>MKIIALRSSLKLAARIAEELKTEPVMPDERRFPDGELYLRYDEDLTGHNIFIIGNTHSDAEVMEMILTLSAIQDYRTKSVNIIAPYYGYARQHQRYKNGEPISSQILTEIYSSYSNSIATVDIHDEKTLSYSKVKFSDLH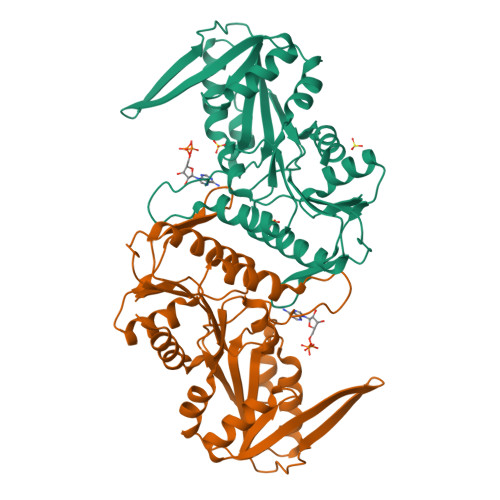ANDAIVRYYKNVDVDYVVSPDDGGLARVADISAKLGKKHFFIEKKRIDDRTVEMKVPNVDVNGKKLLIVDDIISTGGTIAKSSGLLREKGASKIYVSAVHGLFVNGSENKILQNADEIHVTDTVESKFSDISVYQEVCNYIRDIDA[2x]Bacteriophage Sf14 infects the human pathogen Shigella flexneri. Here, we report multiple high-resolution structures of the full Sf14 particle, including symmetric and asymmetric reconstructions of the virion capsid, empty capsid, portal region, tail, and baseplate. Sf14 virions have a spherical icosahedral capsid of 820 Å in diameter, which is connected to a long, contractile tail that is approximately 1205 Å long and an average of 235 Å in diameter, expanding to 315 Å at the baseplate. Overall, phage Sf14 appears to share some similarities to other model phages, but in different combinations: both λ- and T4-like decoration proteins, HK97-like capsid and portal proteins, T4/Mu-like tail fibers, a Mu-like baseplate, and a P2-like tail needle.

However, while many other T = 9 phages have one reported decoration protein, Sf14 appears to have two: one that is present as trimers surrounding each hexamer and a second that is at the center of each quasi 3-fold hexamer. The capsid structure was then resolved to a higher resolution of 3.2 Å via symmetric reconstruction. Each asymmetric subunit contains nine chains of capsid protein gp34, three trimers of decoration protein gp33, and one monomer of decoration protein gp20. The lattice is formed by the N-terminal arm of each gp33 monomer interacting with its neighboring monomer. Within a gp33 trimer, the trimeric interface is stabilized through salt bridges between Asp and Arg on neighboring subunits. The trimer is then anchored to the capsid protein gp34 by additional salt bridges involving gp33 Lys and gp34 Glu. The decoration protein gp20 binds the capsid as a monomer, with the capsid binding domain contained in the N-terminal 118 amino acids, folded into a largely helical bundle. The core of this domain is hydrophobic, while the external surface is enriched in charged and polar residues. This domain is also anchored to the gp34 hexamer by salt bridges, with positively-charged gp20 Arg residues 79 and 107 interacting with three of the six gp34 monomers at Asp 221. The specificity of gp20 for quasi 3-fold hexamers could be due to differences at one of the three gp34 monomers.

>[9x]MLTNSEKSRFFLADLTGEVQSIPNTYGYISGLGLFRSAPQTQTTFLMDLTDWDISLLDAVDRTSRKAETSAPERVRQISFPMMYFKEVESITPDEIQGVRQPGTANELTTEAVVRAKKLMKIRTKFDITREFLFMQALKGKVIDANGVLYADLYKQFDVTKKTIYFDLDNPNSDIDAHIEDLRMHMEDEAKTGTVINGEEIHIVVDRTFFSKLIKHPKIRDAYLAQQTPLAWQQITGSLRTGGTDGVQAHMNRFYYGGVVFVQYNGKFKDKRGKTHTLVSIDGVSDTNVGVGHAFPNVAMLGEANNIFEVAYAPCPKMGYANTLGQELYVFEYEKDRDEGIDFEAHSYMLPYCTRPQLLVDVRSDAE;>MAYQGFTKLGEREPLNDIILWEEITPTGHSRKEYAPVASTEYRVGEVLKADGSKVAAGQEAQADSVCIVNFYADLQLSYHGQLKVVGIYRDAELKDLLKLESGVDAAAVKSALKAKGIDFVPTGL[9x];> MIKAKTYPDFKEFVKDFVANVKAGKRYDFRKYQEAVLPLTYSSPWPESDIPEVTDFNYTPDYTVPFSEELLYSVGAQMRTADFFMDLQYAIINGKDVDTVYCEWLARVKPFSMLNAKLKDSAQPPVITTQPTGGAVNEGSAINLSIVATNATSYQWKKGSSDISGATSATYTKAGAVPADAGSYTCVVTNDVGSTTSDAAVITINPLPVITTQPTSKAVNESSTLTLSVVATGATSYQWKKNGTNISGATSATYSKANAKTTDAGSYTCVVTNAVGSVTSNAATVTINPLPVITVQPQDQDLTVGQTLTISITATGATGYQWRKGNSNISGATSATYTKASVTTADDGNYDCVVTNAVGSVTSHQAKVQVTA>MSTQYETQGYTINNAGRRLVVDPITRIEGHMRCEVNINDQNVITNAVSCGTMFRGLEIILQGRDPRDAWAFVERICGVCTGVHALASVYAIEDAIGIKVPDNANIIRNIMLATLWCHNHLVHFYQLAGMDWIDVLDALKADPRKTSELAQSLSSWPKSSPGYFFDVQNRLKKFVEGGQLGIFRNGYWGHPQYKLPPEANLMGFAHYLEALDFQREIVKIHAVFGGKNPHPNWIVGGMPCAINIDESGAVGAVNMERLNLVQSIITRTADFINNVMIPDALAIGQFNKPWSEIGTGLSDKCVLSYGAFPDIANDFGEKSLLMPGGAVINGDFNNVLPVDLVDPQQVQEFVDHAWYRYPNDQVGRHPFDGITDPWYNPGDVKGSDTNIQQLNEQERYSWIKAPRWRGNAMEVGPLARTLIAYHKGDAATVESVDRMMSALNLPLSGIQSTLGRILCRAHEAQWAAGKLQYFFDKLMTNLKNGNLATASTEKWEPATWPTECRGVGFTEAPRGALGHWAAIRDGKIDLYQCVVPTTWNASPRDPKGQIGAYEAALMNTKMAIPEQPLEILRTLHSFNPCLACSTH[2x];>LENKPRIPVVWIHGLECTCCTESFIRSAHPLAKDVILSLISLDYDDTLMAAAGTQAEEVFEDIITQYNGKYILAVEGNPPLGEQGMFCISSGRPFIEKLKRAAAGASAIIAWGTCASWGCVQAARPNPTQATPIDKVITDKPIIKVPGCPPIPDVMSAIITYMVTFDRLPDV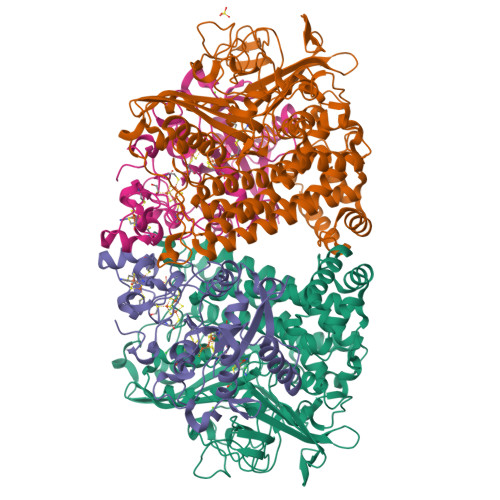DRMGRPLMFYGQRIHDKCYRRAHFDAGEFVQSWDDDAARKGYCLYKMGCKGPTTYNACSSTRWNDGVSFPIQSGHGCLGCAENGFWDRGSFYSRVVDIPQMGTHSTADTVGLTALGVVAAAVGVHAVASAVDQRRRHNQQPTETEHQPGNEDKQARSHHHHHH[2x]> AEPFAKLEQDFGGSIGVYAMDTGSGATVSYRAEERFPLCSSFKGFLAAAVLARSQQQAGLLDTPIRYGKNALVPWSPISEKYLTTGMTVAELSAAAVQYSDNAAANLLLKELGGPAGLTAFMRSIGDTTFRLDRWELELNSAIPSDARDTSS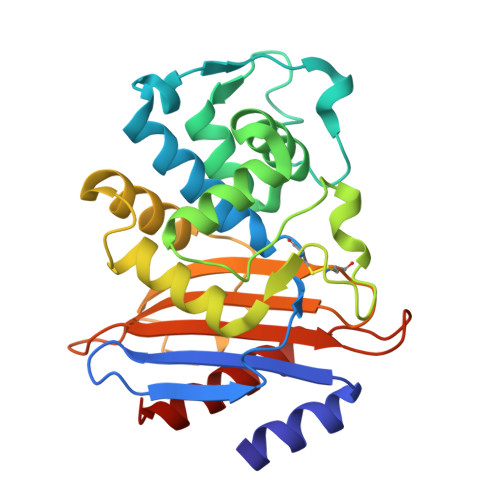PRAVTESLQKLTLGSALAAPQRQQFVDWLKGNTTGNHRIRAAVPADWAVGDKTGTCGVYGTANDYAVVWPTGRAPIVLAVYTRAPNKDDKHSEAVIAAAARLALEGLGVNGQ Here, we identify a protein (CcpS) that is phosphorylated by Stk1 and modulates the activity of phosphatase CpsB in Streptococcus suis, thus linking Stk1 to CPS synthesis. The crystal structure of CcpS shows an intrinsically disordered region at its N-terminus, including two threonine residues that are phosphorylated by Stk1. The activity of phosphatase CpsB is inhibited when bound to non-phosphorylated CcpS. Thus, CcpS modulates the activity of phosphatase CpsB thereby altering CpsD phosphorylation, which in turn modulates the expression of the Wzx-Wzy pathway and thus CPS production.

To gain insights into the architecture and mechanism of CcpS modulates the activity of CpsB, we first solved its structure to 1.6 Å resolution. CcpS also formed a homodimer, each monomer containing four α-helices. Helices were connected by a short loop and a single turn of 310 helix between helices α2 and α3. However, we could not observe the electron density map owing to the highly increased flexibility at the N-terminus of CcpS. Interestingly, two phosphorylation residues Thr4 and Thr7 are included in intrinsically disordered regions (IDRs) of CcpS. Interface residues analysis of CcpS homo-dimer suggested that many amino acids residues were involved in the formation of a dimer. And the amino acids region I73-L81 among helices α4 was contributed to the hydrophobic core, which was similar to the previously reported structures of CcpS homologs. We found that double mutations I73RY80E directly blocked the self-interaction of CcpS. Importantly, we found that the disruption of CcpS homo-dimer structure directly resulted in its dysfunction in regulating the activity of CpsB and thus CPS production. Superimposition of CcpS onto CcpS-T4ET7E folded structure revealed that overall structure was highly similar to each other; however, we can observe that a resolvable structure of N-terminal partial region is significantly different between CcpS and its variant CcpS-T4ET7E (chain A, N-ter).

>MGFTEETVRFRLDDTDKQEISKTLTSVYRSLEEKGYNPINQIIGYVLSGDPAYIPRYNDARNQIRKHERDEIIEELVRYYLKGNGIDL[2x]Energy-coupling factor (ECF)-type transporters mediate the import of micronutrients, such as folate, cobalamin and pantothenate, in the majority of prokaryotes. A tripartite ATP-hydrolysing motor (ECF module), composed of a membrane-embedded scaffold protein (EcfT) and two cytosolic nucleotide-binding proteins or ATPase subunits (often hetero-dimeric - EcfA and EcfA’), forms a functional core complex with a membrane-embedded substrate-translocating protein (S-component). Structural and biophysical analyses of ECF transporter complexes from three different organisms, with different substrate specificities, and from different laboratories revealed that the core complex and minimal functional unit exists in a 1:1:1:1 subunit stoichiometry. Based on these fragmented structural insights, a model for the transport mechanism has been proposed in which a substrate-free solitary S-component with an outward-facing binding site topples within the membrane upon substrate acquisition, associates with the ECF module, and exposes the binding site to the cytosol, thereby moving the substrate across the membrane.

We substituted the catalytic glutamates in the Walker B motif in both ATPase subunits, which are required for ATP hydrolysis, to glutamine. While the purified double mutant (referred to as 2EQcryo) cannot hydrolyse ATP, it is still expected to bind nucleotides, which prompted us to use it for cryo-EM analysis. We obtained a reconstruction of the mutant solitary ECF module 2EQcryo in lipid nanodiscs at 2.6 Å resolution, which shows a markedly distinct conformation from any structure reported so far. In both ATPase subunits, Mg-ATP is now bound and engaged with the signature motif. Compared to the open conformation, the ATPase subunits have moved by ~4 Å towards each other to adopt a closed conformation. Because the two long coupling helices (CH2 and CH3) of the EcfT subunit are anchored into the grooves of the EcfA and EcfA’ subunits, respectively, with conserved X-Arg-X motifs at their C-terminal ends, the closing of the ATPase subunits into a tight dimer forces these C-terminal ends to move towards each other. This movement thrusts the coupling helices from the membrane interface into the lipid environment by ~9 Å, changing their shape from concave to convex. The convex conformation of the coupling helices adopted by the solitary ECF module upon Mg-ATP binding becomes incompatible with the shape of the S-component. Concomitantly, the transmembrane regions of the EcfT subunit that are connected to the coupling helices, undergo a ~13.5 Å rigid body translation and a ~25 Å rotation towards the coupling helices within the lipid nanodisc, thereby moving into the space where S-components dock. The movement of the coupling helices towards the membrane plane upon Mg-ATP binding, shifts the hydrophobic surface boundary, thereby reducing the thickness of the nanodisc density to ~36 Å in this region.

> GSDNIISFDHVTFTYPDSPRPALSDLSFAIERGSWTALIGHNGSGKSTVSKLINGLLAPDDLDKSSITVDGVKLGADTVWEVREKVGIVFQNPDNQFVGATVSDDVAFGLENRAVPRPEMLKIVAQAVADVGMADYADSEPSNLSGGQKQRVAIAGILAVKPQVIILDQSTSMLDPEGKEQILDLVRKIKEDNNLTVISITHDLEEAAGADQVLVLDDGQLLDQGKPEEIFPKVEMLKRIGLDIPFVYRLKQLLKERGIVLPDEIDDDEKLVQSLWQLNSKM;> MAIKFENVSYVYSPGSPLEAIGLDQLNFSLEEGKFIALVGHTGSGKSTLMQHFNALLKPTSGKIEIAGYTITPETGNKGLKDLRRKVSLAFQFSEAQLFENTVLKDVEYGPRNFGFSEDEAREAALKWLKKVGLKDDLIEHSPFDLSGGQMRRVALAGVLAYEPEIICLDQPAAGLDPMGRLEMMQLFKDYQAAGHTVILVTHNMDDVADYADDVLALEHGRLIKHASPKEVFKDSEWLQKHHLAEPRSARFAAKLEAAGLKLPGQPLTMPELADAIKQSLKGGEHE;> MSKIIIGRYLPGTTFVYRVDPRAKLLTTFYFIIMIFLANNWVSYLVISIFGLAYVFATGLKARVFWDGVKPMIWMIVFTSLLQTFFMAGGKVYWHWWIFTLSSEGLINGLYVFIRFAMIILVSTVMTVTTKPLEIADAMEWMLTPLKLFKVNVGMISLVISIALRFVPTLFDQTVKIMNAQRSRGADFNDGGLVKRAKSVVPMLVPLFIDSLEVALDLSTAMESRGYKGSEGRTRYRILEWSKVDLIPVAYCLLLTILMITTRKH N-(5-{3-[(1S,7R,8R,9S)-4-amino-2-oxo-7lambda~4~-thia-3,5-diazatetracyclo[4.3.0.0~1,7~.0~7,9~]nona-3,5-dien-8-yl]propyl}thiophene-2-carbonyl)-L-glutamic 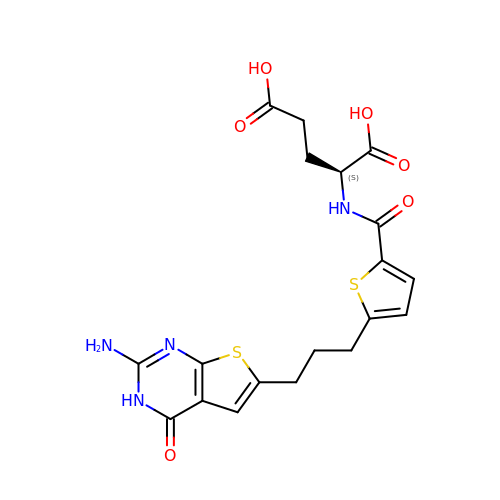acid | C19 H20 N4 O6 S2 | VCNJYHGDMDELAI-LBPRGKRZSA-N>PQVPADVVIDHLSNPNAKLEYKVKFSHKAHASLGTDAAACQKCHHKWDGKSEIGGCATEGCHADTTSFKATEKDPKFLMTAFHSKSPMSCQGCHKEMKTAKKTT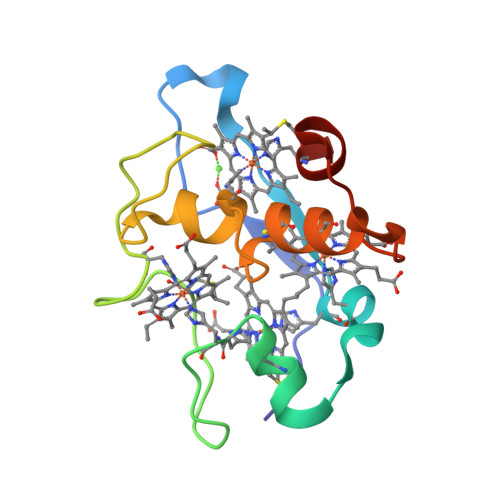GPTACAQCHNQK[2x]>[2x]SHMEQRIL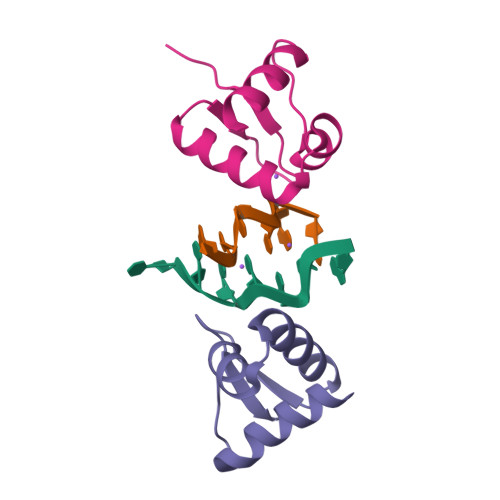KFLEELGEGKATTAHDLSGKLGTPKKEINRVLYSLAKKGKLQKEAGTPPLWKIAVSTQ>GPMGKELKIGVPLRVSYKEFVSQIRGTENMFKGFCIDVFTAAVNLLPYAVPVKFIPYGNGKENPSYTHMVEMITTGNFDGVVGDVAIVTNRTKIVDFTQPYAASGLVVVAPGGTPIKGIESLRERDDPIGYQVGSFAESYLRNELNISESRLVPLGTPEAYAKALKDGPSKGGVAAIVDERPYVELFLSSNCAYRIVGQEFTKSGWGF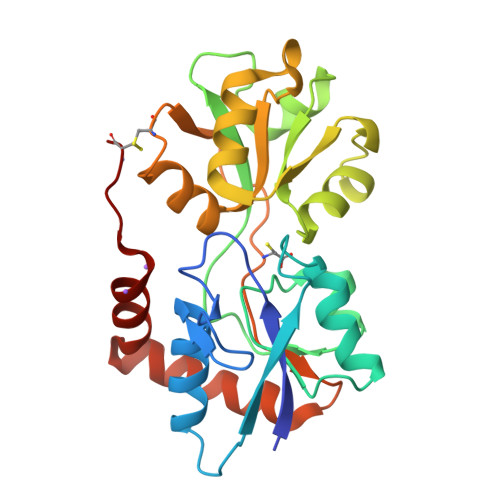AFPRDSPLAIDLSTAILELAENGDLQRIHDKWLMKNACT[4x]>[2x]SMIYAAPGTPGAVVTFKPRYGNYIGGEFVPPVKGQYFTNTSPVNGQPIAEFPRSTAEDIDKALDAAHAAAEAWGRTSVQERSNILLKIADRI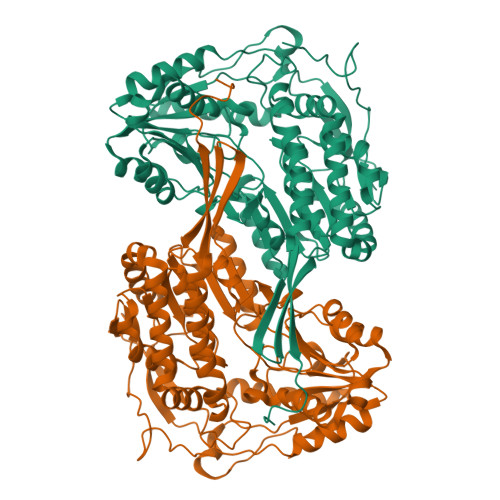EQNLELLAVTETWDNGKAVRETLNADIPLAADHFRYFAGCIRAQEGSAAEINDSTVAYHIHEPLGVVGQIIPWNFPLLMAAWKLAPALAAGNCVVLKPAEQTPLGICVLLELIGDLLPPGVLNVVQGFGREAGEALATSKRIAKIAFTGSTPVGSHILKCAAENIIPSTVELGGKSPNIYFEDIMQAEPAFIEKAAEGLVLAFFNQGEVCTCPSRALVQESIYPAFMEEVLKKVRAIKRGDPLDTETMVGAQASQQQYEKILSYLDIAQQEGAELLAGGSVEKLEGNLASGYYIQPTLLKGHNGMRVFQEEIFGPVVGVTTFKDEAEALAIANDTEYGLGAGLWTRDINRAYRMGRGIKAGRVWTNCYHLYPAHAAFGGYKKSGVGRETHKMMLDHYQQTKNLLVSYDINPLGFF> KPGDVDGNGSINSIDFALMRNYLLGNLKDFPA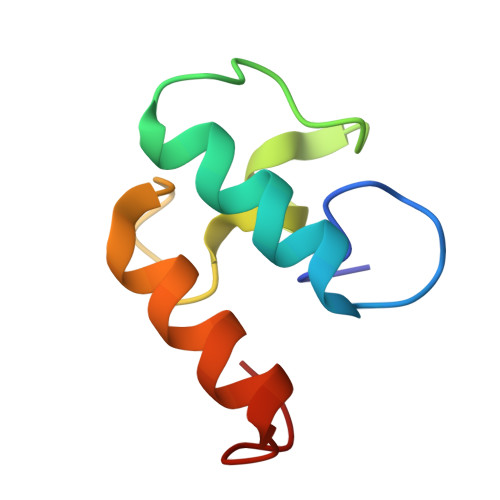EDDIKAGDLNGDKSININDFAIMRMYLLGMITKF> GGLEKDFLPLYFGWFLTKKSSETLRKAGQVFLEELGNHKAFKKELRHFISGDEPKEKLELVSYFGKRPPGVLHCTTKFCDYGKAAGAEEYAQQEVVKRSYGKAFKLSISALFVTPKTAGAQVVLTDQELQLWPSDLDKPSASEGLPPGSRAHVTLGCAADIQPVQTGLDLLDILQQVKGGSQGEAV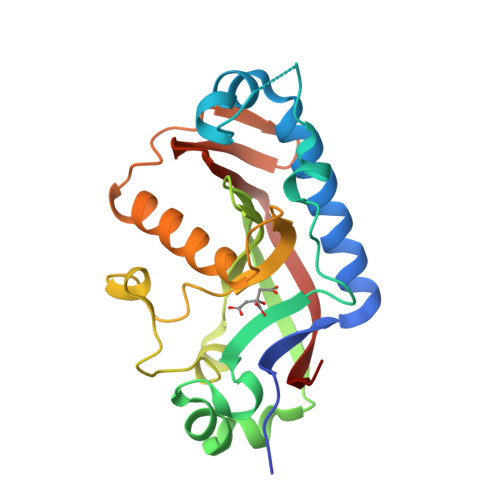GELPRGKLYSLGKGRWMLSLTKKMEVKAIFTGYYG> MFQQLSARLQEAIGRLRGRGRITEEDLKATLREIRRALMDADVNLEVARDFVERVREEALGKQVLESLTPAEVILATVYEALKEALGGEARLPVLKDRNLWFLVGLQGSGKTTTAAKLALYYKGKGRRPLLVAADTQRPAAREQLRLLGEKVGVPVLEVMDGESPESIRRRVEEKARLEARDLILVDTAGRLQIDEPLMGELARLKEVLGPDEVLLVLDAMTGQEALSVARAFDEKVGVTGLVLTKLDGDARGGAALSARHVTGKPIYFAGVSEKPEGLEPFYPERLAGRILGM;> GFFDRLKAGLAKTRERLLKAIPWGGNLEEVLEELEMALLAADVGLSATEEILQEVRASGRKDLKEAVKEKLVGMLEPDERRATLRKLGFNPQKPKPVEPKGRVVLVVGVNGVGKTTTIAKLGRYYQNLGKKVMFCAGDTFRAAGGTQLSEWGKRLSIPVIQGPEGTDPAALAYDAVQAMKARGY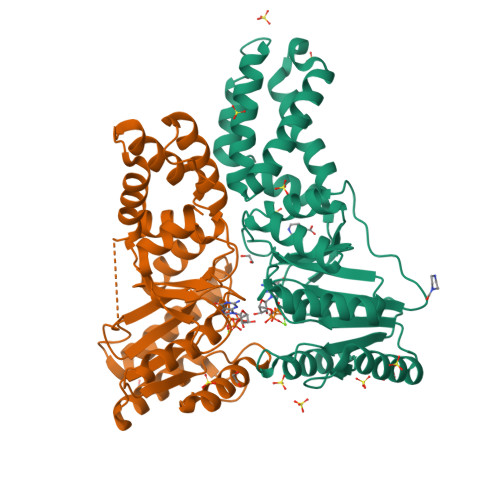DLLFVDTAGRLHTKHNLMEELKKVKRAIAKADPEEPKEVWLVLDAVTGQNGLEQAKKFHEAVGLTGVIVTKLDGTAKGGVLIPIVRTLKVPIKFVGVGEGPDDLQPFDPEAFVEALLED> MDLTVEPNLHSLITSTTHKWIFVGGKGGVGKTTSSCSIAIQMALSQPNKQFLLISTDP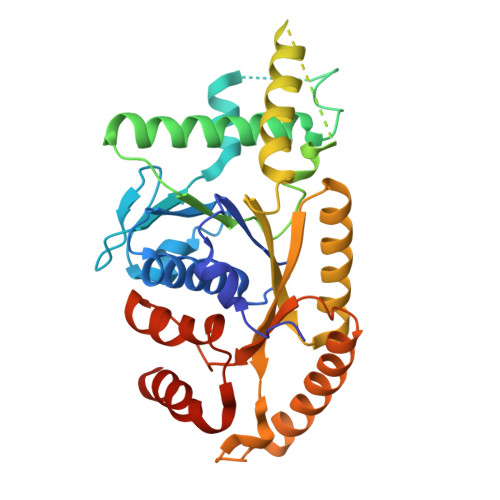AHNLSDAFGEKFGKDARKVTGMNNLSCMEIDPSAALKDMNDMAVSRANNNGSDGQGDDLGSLLQGGALADLTGSIPGIDEALSFMEVMKHIKRQEQGEGETFDTVIFDTAPTGHTLRFLQLPNTLSKLLEKFGEITNKLGPMLNSFMGAGNVDISGKLNELKANVETIRQQFTDPDLTTFVCVCISEFLSLYETERLIQELISYDMDVNSIIVNQLLFAENDQEHNCKRCQARWKMQKKYLDQIDELYEDFHVVKMPLCAGEIRGLNNLTKFSQFLNKEYNPITDGKVIYELEDKELEHHHHHH2-(5-{[({3-[(1R)-1-[({(2S)-1-[(2S)-2-[(1S)-cyclohex-2-en-1-yl]-2-(3,4,5-trimethoxyphenyl)acetyl]piperidin-2-yl}carbonyl)oxy]-3-(3,4-dimethoxyphenyl)propyl]phenoxy}acetyl)amino]methyl}-6-hydroxy-3-oxo-3H-xanthen-9-yl)benzoic acid | C63 H64 N2 O15 | 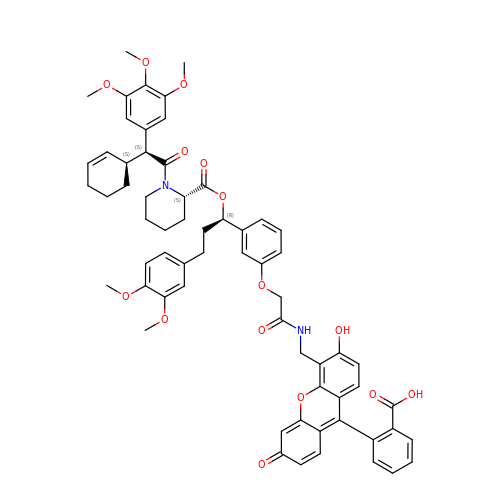VYEGSGNDADHBPR-OQAOPSLVSA-N(S)-10-[(DIMETHYLAMINO)METHYL]-4-ETHYL-4,9-DIHYDROXY-1H-PYRANO[3',4':6,7]INOLIZINO[1,2-B]-QUINOLINE-3,14(4H,12H)-DIONE | 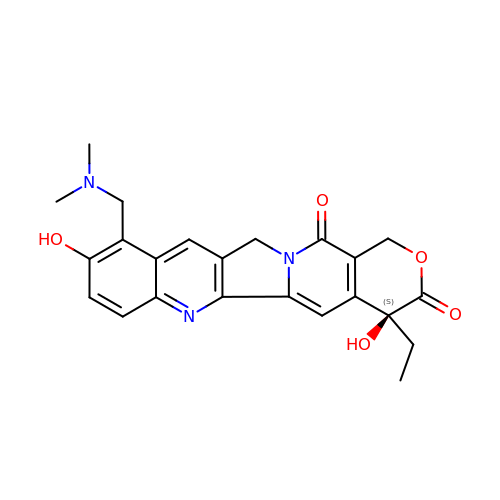C23 H23 N3 O5 | UCFGDBYHRUNTLO-QHCPKHFHSA-N Like the TET proteins, T7H is also a Fe2+ and α-KG dependent dioxygenase. Here we report the crystal structures of N. crassa T7H (NcT7H) in apo form, in α-KG-bound form and in complexes with α-KG and T, 5hmU or 5fU. Similar to other α-KG dependent dioxygenases, NcT7H adopts a variation of double-stranded β-helix (DSBH) fold as the core. The active site of NcT7H is located at the front end (opposite to the back end) of the DSBH core and partially covered by the α10 helix at the C-terminus.

Crystallization of a C-terminal truncated NcT7H (residues 1–299, NcT7HΔC) alone yielded the apo-form crystals. The Crystal structure of the apo NcT7HΔC was solved by the SAD method at 2.3 Å resolution. The asymmetric unit contains one NcT7HΔC molecule, which is well defined except four surface exposed regions (residues 95–116, residues 198–207, residues 278–282, and residues 296–299). There is a metal ion bound at the active site, which is provisionally interpreted as calcium as the ICP-AES (inductively coupled plasma atomic emission spectroscopy) analysis revealed that calcium is the most abundant metal in the protein solution and the structure refinement yielded a reasonable B-factor. Since no divalent metal ion was added in the purification and the crystallization solution, the bound Ca2+ is presumably co-purified with the enzyme. In the apo NcT7HΔC structure, the Ca2+ is coordinated by three strictly conserved residues His214, Asp216 and His271, which constitute the characteristic HXD/E…H motif of α-KG dependent dioxygenases, and three water molecules in an octahedral geometry. The binding and coordination geometry of the Ca2+ and Ni2+ may resemble these of the Fe2+ to some extent. Indeed, our crystallization experiments show that co-crystallization of NcT7HΔC with α-KG and the substrates yielded only the α-KG-bound form (data not shown). In addition, our biochemical data show that NcT7HΔC could not catalyse the oxidation reaction of T, 5hmU or 5fU. The structural and biochemical data together indicate that the C-terminal region of NcT7H is essential for the substrate binding and catalysis.

> GSMEKAAVNEDGLVIPLIDFSKFLEGDETLKLETAKAILHGFQTAGFIYLKNIPIQPDFREHVFNTSAKFFKLPKEKKLEVGWTTPEANRGYSAPGREKVTQLTDPAEIEKIRSAAPDIKESYEIGREDEPGHPNPWPAEQDDLVGFKSTMNNFFDQCKALHIEVMRAIAVGMGIDANYFDSFVDVGDNILRLLHYPAVKSEVFKINPGQVRAGEHTDYGSITLLFQDSRGGLQVKSPNGQFIDATPIENTVVVNAGDLLARWSNDTIKSTVHRVVEPPKQEDVHPPRYSIAYFCNPNHKSLEHHHHHH> QGAHDLKTFSSKSE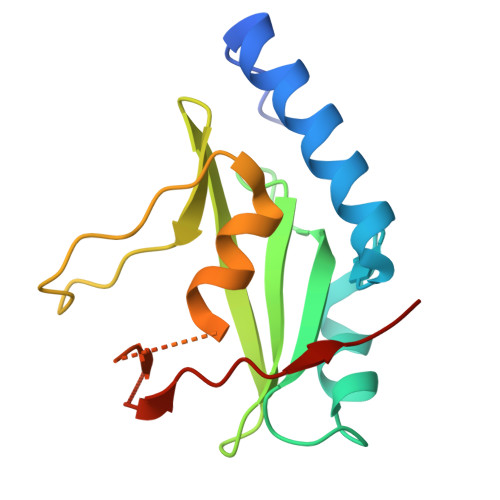YQLVVNAVRKLQESGFYWSAVTGGEANLLLSAEPAGTFLIRDSSDQRHFFTLSVKTQSGTKNLRIQCEGGSFSLQSDPRSTQPVPRFDCVLKLVHHYMGSGSGSGSRAYYIYSGGEKIPLVLSRPLSSN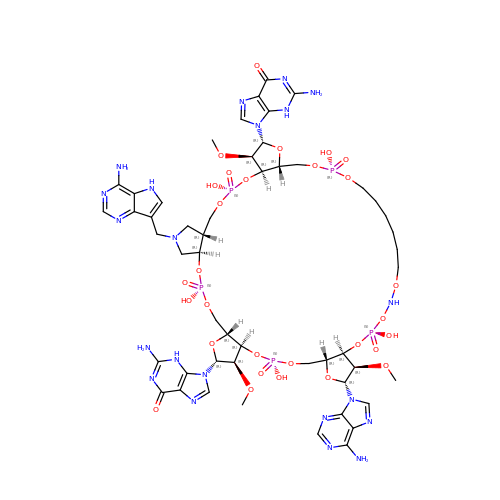9,9'-{(2R,3R,3aR,5S,7aR,9R,10R,10aR,12S,23R,25aR,27R,28R,28aR,30S,32aR,35aR,37S,39aR)-9-(6-amino-9H-purin-9-yl)-34-[(4-amino-5H-pyrrolo[3,2-d]pyrimidin-7-yl)methyl]-5,12,23,30,37-pentahydroxy-3,10,28-trimethoxy-5,12,23,30,37-pentaoxidotetracosahydro-2H,7H,25H-trifuro[3,2-f:3',2'-l:3'',2''-x]pyrrolo[3,4-r][1,3,5,9,11,15,17,21,23,27,29,2,4,10,16,22,28]undecaoxazapentaphosphacyclopentatriacontine-2,27-diyl}bis(2-amino-3,9-dihydro-6H-purin-6-one) | C51 H72 N21 O29 P5 | UYGVCRAKTIGHOS-DFLHJNKYSA-N>[45x]AEGDDPAKAAFDSLQA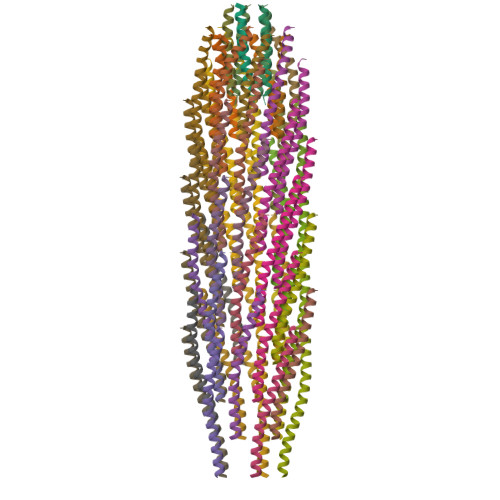SATEMIGYAWAMVVVIVGATIGIKLFKKFTSKAS;>[5x]MEQVADFDTIYQAMIQISVVLCFALGIIAGGQR;>[5x]MSVLVYSFASFVLGWCLRSGITYFTRLMETSS> AERSELTIHPKEFTTFVRNFNPFLGATNLHTTTDFIYEPLVVFNEMHGNTPVFRLAENFQMSDDLMSVTFDIRKGVKWSDGEAFTADDVVYSFNLVKEKPELDQSGINSWVTGVEKVNDYQVKFRLSEANSNVPYEIAKVPVVPKHVWSKVKDPSTFTNENPVGSGPFTVIDTFTPQLYIQCENPNYWDAANLDVDCLRVPQIANNDQFLGKVVNGEMDWTSSFVPDIDRTYAAASPKHHYWYPPAGTQAFVVNFKNPDAAKNEALTNVDFRRAFSMALDRQTIIDIAFYGGGTVNDFASGLGYAFEAWSDEKTHDKFKAYNSYNAEGAKKLLAKAGFKDV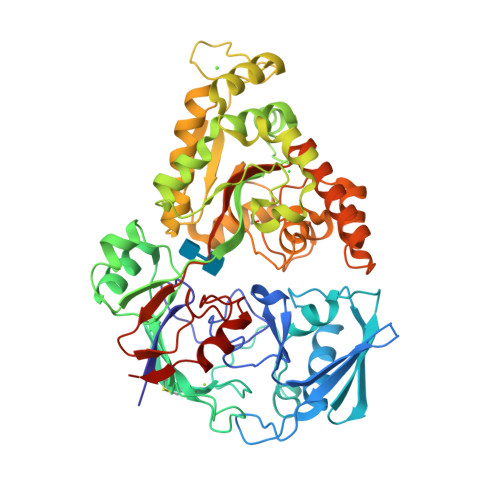NKDGFVDTPSGKSFELLIQSPNGWTDFNNTVQLAVEQLAEVGIKARARTPDFSVYNQAMLEGTYDVAYTNYFHGADPYTYWNSAYNSALQSGDGMPRFAMHFYKNEKLDGLLNSFYKTADKQEQLEIAHGIQQIIAQDQVTIPVLSGAYMYQYNTTRFTGWWNEENPKGRPNIAAGIPERLLHVLDLKPVKHHHHHH>MKLSGVELRRVQMPLVAPFRTSFGTQSVRELLLLRAVTPAGEGWGECVTMAGPLY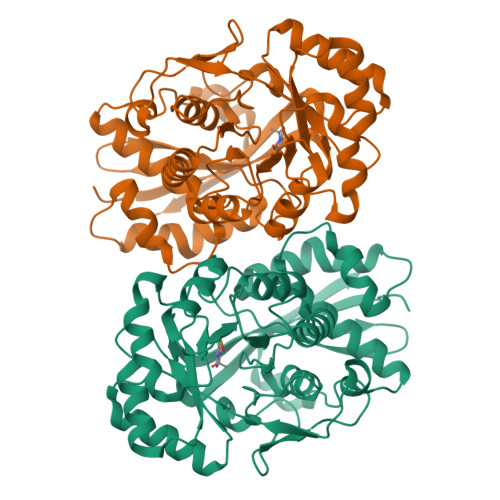SSEYNDGAEHVLRHYLIPALLAAEDITAAKVTPLLAKFKGHRMAKGALEMAVLDAELRAHERSFAAELGSVRDSVPCGVSVGIMDTIPQLLDVVGGYLDEGYVRIKLKIEPGWDVEPVRAVRERFGDDVLLQVDANTAYTLGDAPQLARLDPFGLLLIEQPLEEEDVLGHAELARRIQTPICLDESIVSARAAADAIKLGAVQIVNIKPGRVGGYLEARRVHDVCAAHGIPVWCGDMGETGLGRAANVALASLPNFTLPGDTSASDRYYKTDITEPFVLSGGHLPVPTGPGLGVAPIPELLDEVTTAKVWIGS[4x]>[2x]MNTSLFKQERQKYIPKLPNILKKDFNNISLVYGENTEAIQDRQALKEFFKNTYGLPIISFTEGESSLSFSKALNIGIILSGGPAPGGHNVISGVFDAIKKFNPNSKLFGFKGGPLGL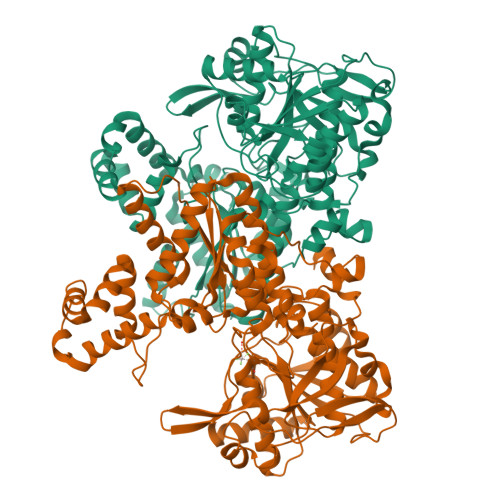LENDKIELTESLINSYRNTGGFDIVSSGRTKIETEEHYNKALFVAKENNLNAIIIIGGDDSNTNAAILAEYFKKNGENIQVIGVPKTIDADLRNDHIEISFGFDSATKIYSELIGNLCRDAMSTKKYWHFVKLMGRSASHVALECALKTHPNICIVSEEVLAKKKTLSEIIDEMVSVILKRSLNGDNFGVVIVPEGLIEFIPEVKSLMLELCDIFDKNEGEFKGLNIEKMKEIFVAKLSDYMKGVYLSLPLFIQFELIKSILERDPHGNFNVSRVPTEKLFIEMIQSRLNDMKKRGEYKGSFTPVDHFFGYEGRSAFPSNFDSDYCYSLGYNAVVLILNGLTGYMSCIKNLNLKPTDWIAGGVPLTMLMNMEERYGEKKPVIKKALVDLEGRPFKEFVKNRDKWALNNLYLYPGPVQYFGSSEIVDEITETLKLELFK> MPEDILVDIKRDYVLSKLRDNERIDGRGFDEFRKVEIIPNVIEKAEGSALVKLGDTQVVVGVKMQPGEPAPDTPDRGVIIVNAELVPLASPTFEPGPPDENSIELARVVDRGIRESEAVDLS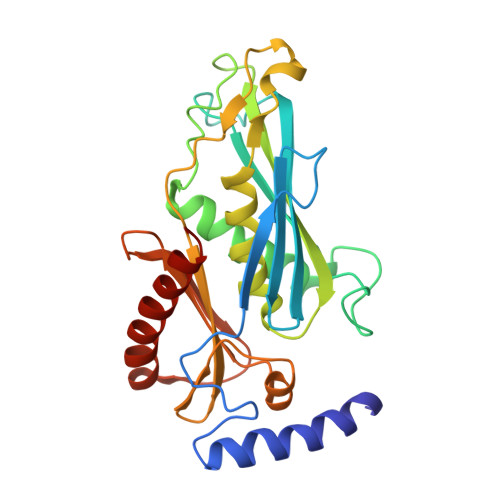KLVIEEGEKVWIVFVDIHALDDDGNLLDASALAAIAALMNTKVPAERFDLGEDYLLPVRDLPVSVTSLIVGNKYLVDPSREEMSVGDTTLTITTDKDDNVVAMQKSGGYLLDEKLFDELLDVSINCARKLREKFKEI> STAFVDQDKQMANRLNLSPLERSKIEKQYGGATTLAFISNKQQELAQILSRADILKIASYDCAAHALQAVLDCGPMLGKRGFSQSDIVKIAGNIGGAQALQAVLDLESMLGKRGFSRDDIAKMAGNIGGAQTLQAVLDLESAFRERGFSQADIVKIAGNNGGAQALYSVLDVEPTLGKRGFSRADIVKIAGNTGGAQALHTVLDLEPALGKRGFSRIDIVKIAANNGGAQALHAVLDLGPTLRECGFSQATIAKIAGNIGGAQALQMVLDLGPALGKRGFSQATIAKIAGNIGGAQALQTVLDLEPALCERGFSQATIAKMAGNNGGAQALQTVLDLEPALRKRDFRQADIIKIAGNDGGAQALQAVIEHGPTLRQHGFNLADIVKMAGNIGGAQALQAVLDLKPVLDEHGFSQPDIVKMAGNIGGAQALQAVLSLGPALRERGFSQPDIVKIAGNTGGAQALQAVLDLELTLVEHGFSQPDIVRITGNRGGAQALQAVLALELTLRERGFSQPDIVKIAGNSGGAQALQAVLDLELTFRERGFSQADIVKIAGNDGGTQALHAVLDLERMLGDRGFSRADIVNVAGNNGGAQALKAVLEHEATLNERGFSRADIVKIAGNGGGAQALKAVLEHEATLDERGFSRADIVRIAGNGGGAQALKAVLEHGPTLNERGFNLTDIVEMAANSGGAQALKAVLEHGPTLRQRGLSLIDIVEIASNGGAQALKAVLKYGPVLMQAGRSNEEIVHVAARRGGAGRIRKMVAPLLERQGGSEFELENLYFQGELRRQASALE

In a search for putative DNA-binding domains, BurrH, a protein that recognizes a 19 bp DNA target, was identified. Here, its apo and DNA-bound crystal structures are reported, revealing a central region containing 19 repeats of a helix–loop–helix modular domain (BurrH domain; BuD), which identifies the DNA target by a single residue-to-nucleotide code, thus facilitating its redesign for gene targeting. We identified BurrH in Burkholderia rhizoxinica, a symbiotic bacterium found in the cytosol of Rhizopus microspores. Each BuD repeat is composed of 33 residues, only eight of which are strictly conserved between the repeats.

The DNA bearing A, A and T at positions 4, 12 and 13, respectively, displayed the highest affinity and was the only one that yielded crystals of the BurrH–DNA complex; consequently, we performed the rest of the characterization using this target sequence. The models were refined to 2.21 and 2.65 Å resolution, respectively. BurrH shrinks 23 Å along the longitudinal axis wrapping the DNA molecule, which displays an almost unperturbed B-form. The electrostatic potential of BurrH shows two electropositive stripes running along the protein which contact the phosphate backbones of the double helix. In contrast to the TALEs, which only interact with their coding strand, the presence of the second electropositive stripe on the surface of BurrH determines the interaction of the repeat array with both strands of its DNA target. The 4th, 12th and 13th repeats in BurrH show new associations (Thr–A and Arg–G) involving bases in the coding and noncoding strands, respectively. Thr193 and Thr457 in BurrH associate with A+4 and A+12 in the coding strand. The guanidinium group of Arg490 builds a network of interactions with A+14 in the coding strand and T+6 and G+5 in the noncoding strand. In the final repeat the side chain of Arg753 disrupts the A–T pair, generating a hydrogen bond to T−1 in the noncoding strand and a cation–π interaction between its guanidinium group and the ring of T+20 in the coding strand. Therefore, all BurrH arginines present at the 13th position of the BuD repeat interact with the noncoding-strand bases, suggesting that these amino acids may play an important role in DNA target recognition and could be employed to restrict the interaction of the protein with double-strand nucleic acids.>PTFFSTMNTSFSDIELLEDSGIPTEAFLASCYAVVPVLDKLGPTVFAPVKMDLVGNIKKVNQKYITNKAKFTTLQKIVLHEVEADVAQVRNSATEALLWLKRGLKFLKGFLTEVKNGEKDIQTALNNAYGKTLR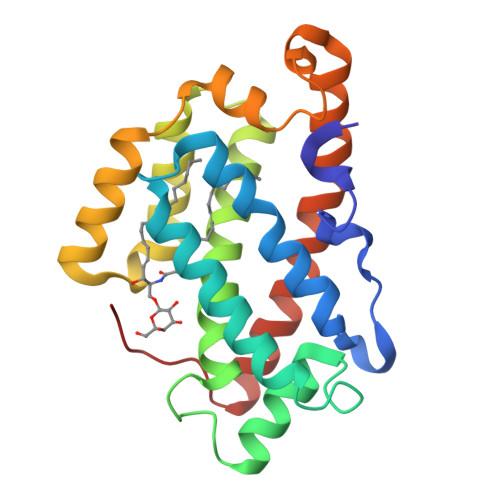QHHGWVVRGVFALALRAAPSYEDFVAALTVKEGDHQKEAFSIGMQRDLSLYLPAMEKQLAILDTLYEVHGLESDEVV[2x]2,4-dibromo-6-{[(2-nitrobenzene-1-carbonyl)amino]methyl}phenyl 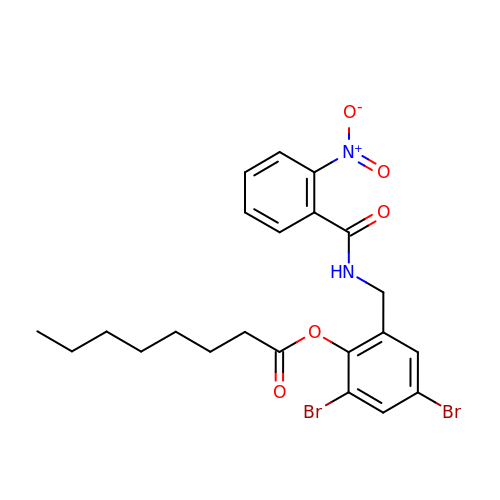octanoate | C22 H24 Br2 N2 O5 | NDEWIQZBBTYPHA-UHFFFAOYSA-N> MARIRHEKEKLLADLDWEIGEIAQYTPLIVDFLVPDDILAMAADGLTPELKEKIQNEIIENHIALMALE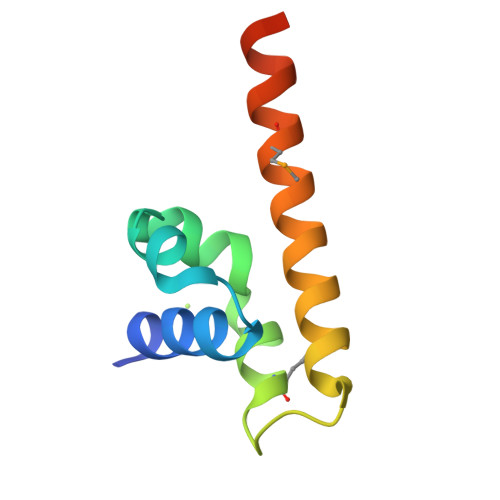EYSSLEHHHHHH(3Z)-3-iminocyclohex-1-ene-1-carboxylic acid | C7 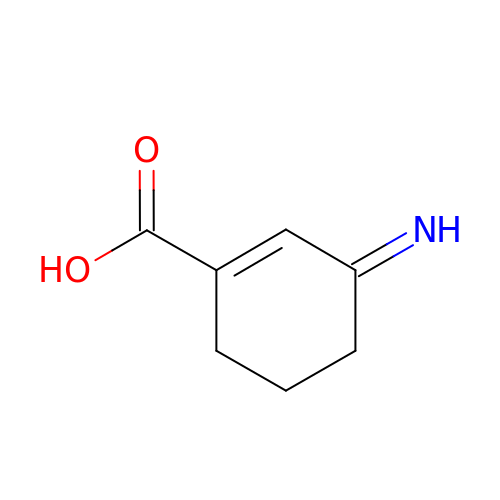H9 N O2 | QYQCRKOROWCYTP-VURMDHGXSA-N>[6x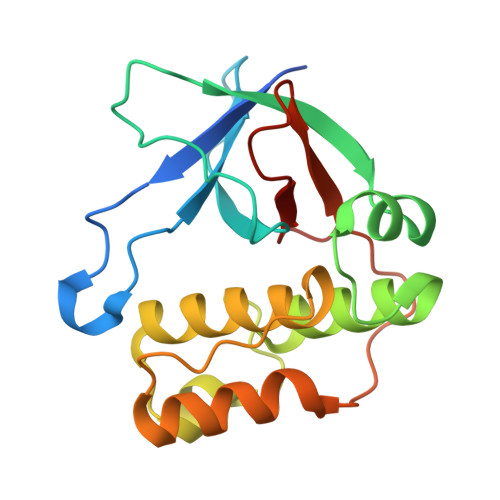]GPSPTGGLQTSTKYKGYTLLDKYPKEDDFRDAIYIEDMDNNDTSSVVYCFNVTKATPTFKGSVVKVLYNEQFGSSKLFTEKAIKPRVKGDELKNSVLRVIYNGYPSNALGIKEKYQLTEGQFRKLTQRAVWNFTDSNLSLDKLSQKEIDALNELINAKNAIPDNLVLNLYLPDDSYYQNLLGTKFVTP>MIAGSMVALVTPFDAQGRLDWDSLAKLVDFHLQEGTNAIVAVGTTG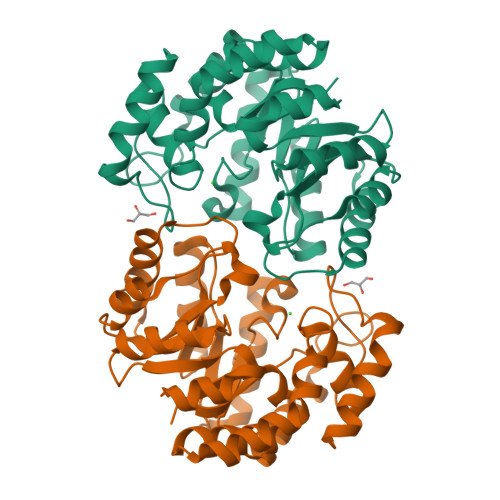ESATLDVEEQIQVIRRVVDQVKGRIPVIAGTGANSTREAVALTEAAKSGGADACLLVTPYYNKPTQEGMYQHFRHIAEAVAIPQILYNVPGRTSCDMLPETVERLSKVPNIIGIKEATGDLQRAKEVIERVGKDFLVYSGDDATAVELMLLGGKGNISVTANVAPRAMSDLCAAAMRGDAAAARAINDRLMPLHKALFIESNPIPVKWALHEMGLIPEGIRLPLTWLSPRCHEPLRQAMRQTGVLA[2x]>[2x]MTDRYEQINDYIEALLKPRPDNVKRLEAYAEEHHVPIMEKAGMEVLLQ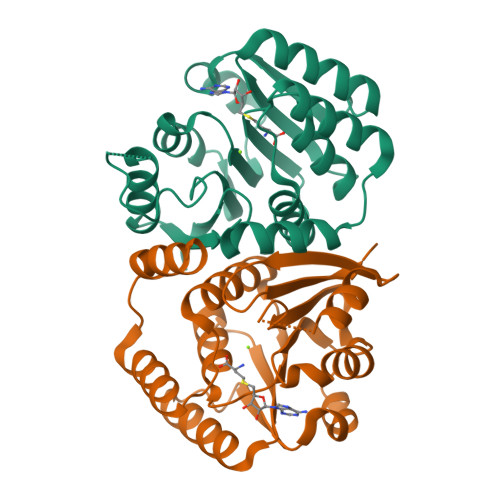ILSVKQPKKILEIGTAIGYSAIRMALELPSAEIYTIERNEKRHEEAVNNIKEFQLDDRIHVFYGDALELADAVHVTAPYDVIFIDAAKGQYQNFFHLYEPMLSPDGVIITDNVLFKGLVAEDYSKIEPKRRRRLVAKIDEYNHWLMNHPDYQTAIIPVGDGLAISKKKRGHHHHHHG> TLIELMIVVAIIGILAAIAIPQYQNYIAKSQVSRVMSETGSLKTVIETCILDGK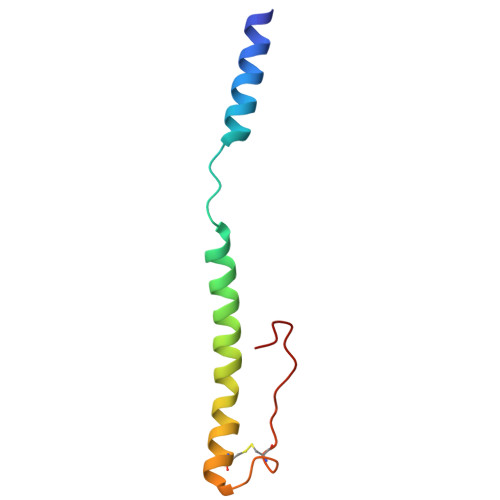TAANCELGWTNSNLLG{1-(ethylsulfonyl)-3-[4-(2-{[3-fluoro-4-(1-methylpiperidin-4-yl)phenyl]amino}-7H-pyrrolo[2,3-d]pyrimidin-4-yl)-1H-pyrazol-1-yl]azetidin-3-yl}acetonitrile 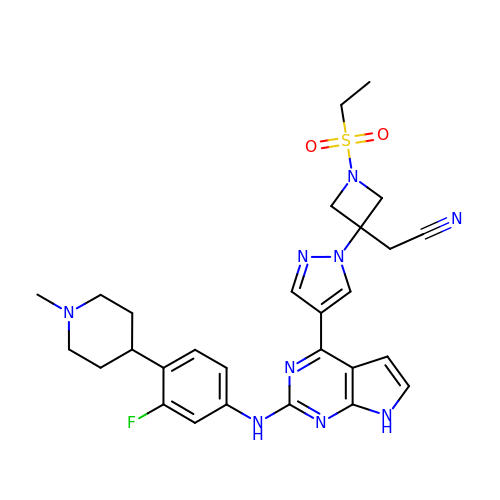| C28 H32 F N9 O2 S | KODVAIZRONHLFN-UHFFFAOYSA-N>MAKTLFRLVSFAAALSTVLGHAVVTVPTPRGAGPYYTQRCGETYAVYMEKDKAGPIENGVAKAGSELGCNPFLCRGYQYEDNEAVEYEPGQVIDFHVDLIAGHHPGYANVSIVDLEANKIIGDPLRSWDDYPNATATTPRSDIDFNVTIPNTLGT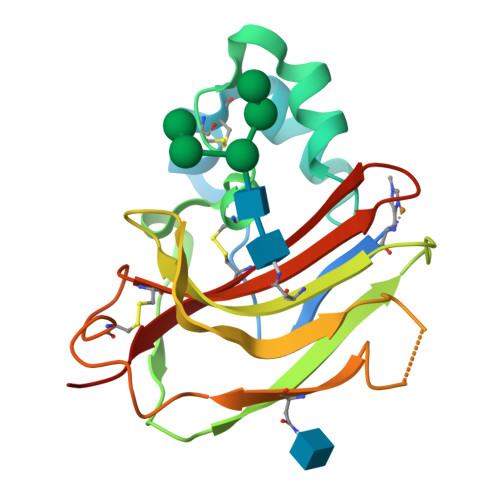ACSTGGKCAIQWYWYASGNKQSYESCVDFYVKA[3x]> QGPRDIALGSSVVSIKNQALGGSLLHSHIQTYPDGSNQQQVTCYGYKDANNEWFFNRERGLPSWSENETDIEYLKPGTSYRLVHKSTGRNLHTHPVAAPVSKTQWEVSGYGDNVVGDNKDNWV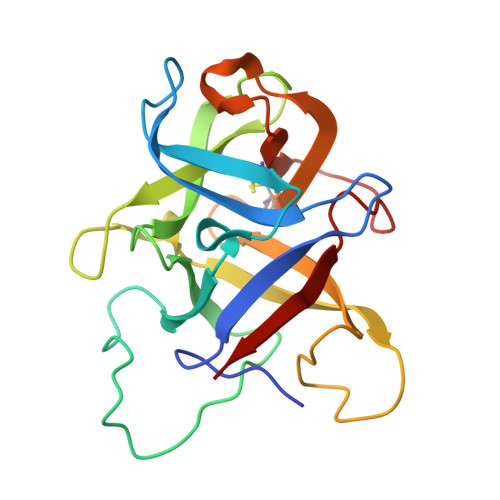IEIMDQRGDEDPEKLHTLTTSFRIKNLEMGCYLAQTGNSLPEWGFRQQEVVCMKNPFKRDKRTWWNIETHENE> MAKENTQQKEIKRQPAVELAVFNLNSVTDVADLQMIASQVQLYLQVCGNTTLEQIKSKANITTVANIFALTGSVLDLMLYATDKKTGDAAVQRGALLAANLIGLFSEPNNEAHARMALRPMFGLMAECLYRENGKIKETDIKRLGLHLNAMIAGDLENFLKETQAKLSSLLISATTLGVTILQSMATPATGINAGITTAAGASAEKRDPKLKFTNWAVPLIDLLGKPSQANLTPKIQPNITSRLQQEATQAIAALSQTLQQQANAGQKYTLAWLLQETLKAIQALENKGNASVPINQTGEYERHTKGDTLEFVSLQADALNAPPCEGADSQSGKSISYS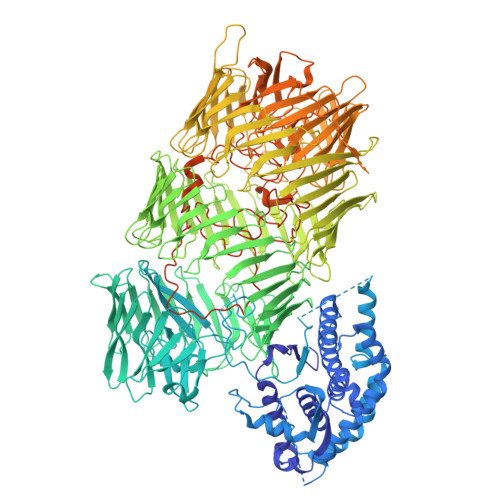IGAERVQHADFYLPKIGFSFIRQYNSQMDEFDQSMVGARWMMPFSNMIQQNAQGYLFIDSKGRKHQLPVSIIFETYEVPYEGWIIKPLKNGELILDFGGEWRSHFQSFDGGKNYYLVKKMNETSQEEILLEYLLLDHIAYLKVINFKLKQAEYELKFAFNEQVKIIAVFLDDKAEPLARYEYDTQGNLIKAIDQNGHTRTYEYNQFHQLTRYTDRTGRGQNIRYESTEAKAKAIEEWADDGSFHTKLKWHPRLRQVAVYDAYDVPTYYYFDLDGFTYRTRLADGRESWYSRDGKKRITRQIDFDGRETQQEYNDQDQLVKIVQPNGGIIRFAYNKQGNLVEIKDPEGSIWKREYDENRNVSKEINPLGHITQYKYNNDNQLVEVIDAKGGVKKIQYNELGQMISYTDCSGKSSTWEYDEDGALTAEQTANNKVVQYFYSTKGRDKGQLQSIIYPDGLKEYFEHDEEGRLLKHTDTKGLVTEYKYNQVGLLEQRIDANRHSVAYQWDKQGRIQKLINQNQAEYLFGYNPYGYLIREQAFDGEEKHYSYNENGRLFQIRRPNILTQFDYYADGQIASKSFTHLHTGQKQTEQFDYNLNSQLSRASNEVSQIDLYRNALGQLVREHQHYKIPELKPLTAVLHYEYDELGNLIKTIRPDGHTLNHLVYGSGHIYAIGLNNQEVVSFQRDDLHRETTRLLANGLMQTKQYNDVGLLSSQFIQPEQETQDYLQYQAHRKYHYDKNYLLSQVEDSRLGKLNYQYDPIGRLIAAQSLHKTESFNFDPAGNLIDSESVLSPAQIKNNLIKSYKGKHYQYDVQGNVTEIIQAGKNLKLTWDNQNRLIRSDNNGLVTEYGYDVFGRRLYKKTAKELTLFGWDGDLMIWESFKSAQTNYTKHYIYEPDSFVPLLQAGYKDFIQLIETPDYQEYQTKPYSIYKDPVWNRNLGKERTALEQFTFYHCDQVGTPQTMTNIRGECVWEILQDTWGAVSQIKALNQDNPFEQNNLRFQGQYYDRETELHYNRYRYYEPHSARYVSKNPIGLEGGMNTSSYVSDPNQWINPKGLNSFNYGEMFGIPASAQSGLAYQGQRNYECYAETGELCKIKVPPLFDYVACSGGGLGIGVGFVKNQWTGEYYISGSKDSLLIPVAKSVAQNKQFSAKDLAGASCVGGNIHNIPSYTKTTMTMGEITNEFVSGASVTVGGGAYGAVANVVVPLVSKSSPVKGTWASELGVGTPGFNVGVSGTVSVDTILDAVKPSKKHHHHHH4-(2-CARBOXYETHYL)(HYDROXY)PHOSPHORYL]-3-OXOBUTANOIC ACID | C7 H11 O7 P | 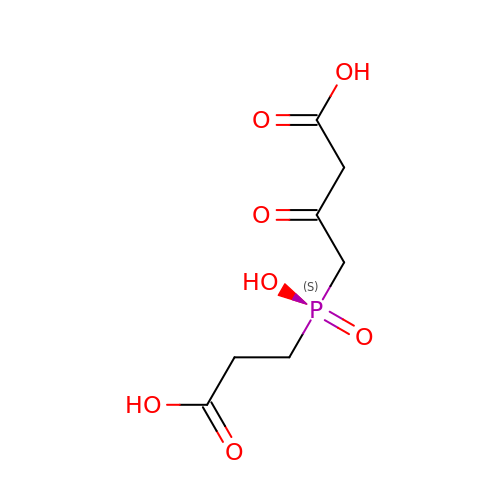YKFFQOHPUCXFLE-UHFFFAOYSA-N2,5,6-triaminopyrimidin-4-ol 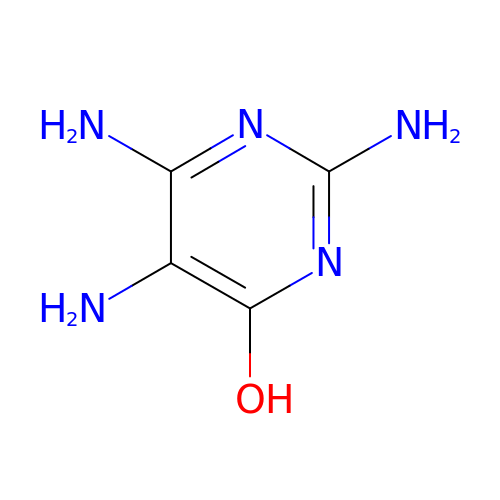| C4 H7 N5 O | SYEYEGBZVSWYPK-UHFFFAOYSA-N> LRYHGDPMPCPKEDTPNSVWEPAKAKYVFRDVVQITCLDGFEVVEGRVGATSFYSTCQSNGKWSNSKLKCQPVDCGIPESIENGKVEDPESTLFGSVIRYTCEEPYYYMENGGGGEYHCAGNGSWVN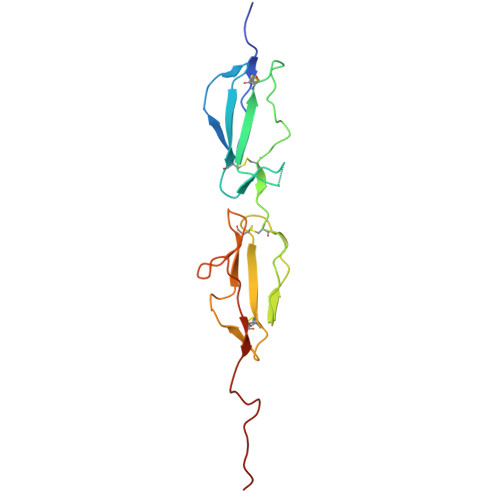EVLGPELPKCVPVCGVPREPFEEKQ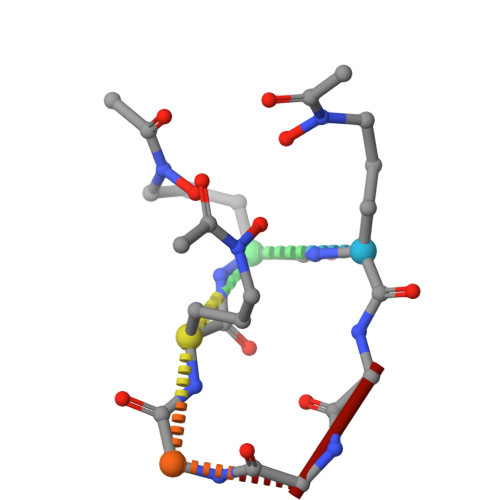> AAAGGG> SLTRIDHIGIACHDLDATVEFYRATYGFEVFHTEVNEEQGVREAMLKINDTSDGG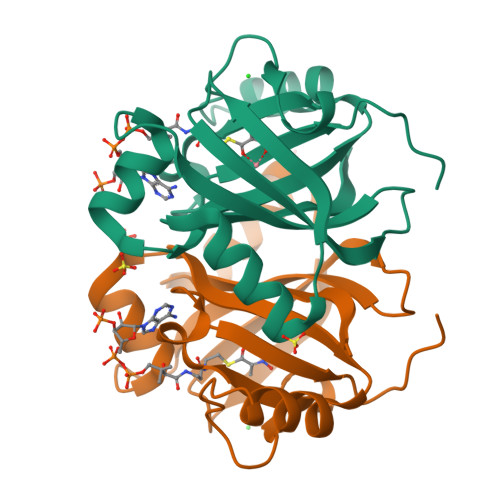ASYLQLLEPTREDSAVGKWLAKNGEGVHHIAFGTADVDADAADIRDKGVRVLYDEPRRGTMGSRITFLHPKDCHGVLTELVTSAAVESPEH> SHMSELSEIDSVAGVTIYSVDGEPKSFVYKAGFAIDADGAPNAYAPNNGGTDFTANGGDDQGGDWWGGPVDAEGYPIKQKIFDPFPGYYVSATAHFNPAYSEDSPYRYIDSNSIPFIVLPGNHSNGAKLGDVALVYNEKTGDNCYAIYGDVGPSSKIGQGSVRLAQALKIDDNPKAGGTESRIVVTLVFPGSVGKWETPKRWFSHANQLTKAWGGLSRLKTLSDQ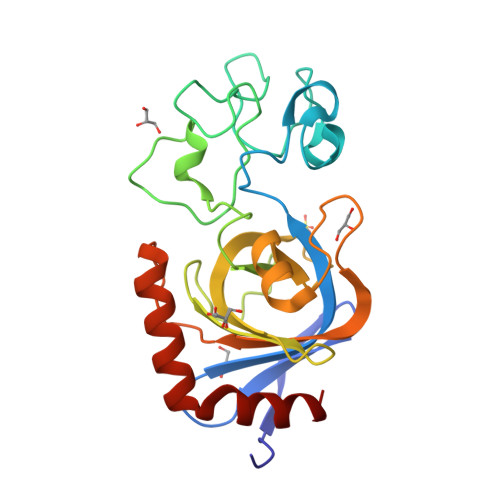L>MHHHHHHHHGSENLYFQSVKLIESKEAFQEALAAAGDKLVVVDFSATWCGPCKMIKPFFHSLCDKYSNVVFLEVDVDDCQDVAADCEVKCMPTFQFYKKGQKVGEFSGANKEKLEATITEFA[2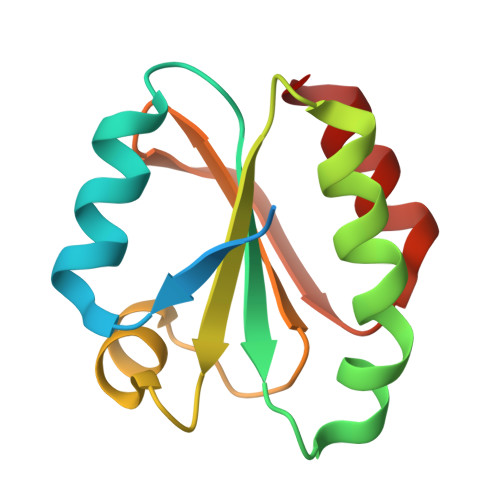x]> ETGLQPLPPTAFTPNGTYLQHLARDPTSGTLY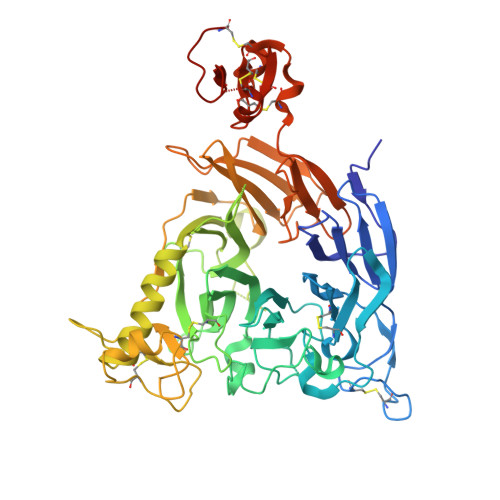LGATNFLFQLSPGLQLEATVSTGPVLDSRDCLPPVMPDECPQAQPTNNPNQLLLVSPGALVVCGSVHQGVCEQRRLGQLEQLLLRPERPGDTQYVAANDPAVSTVGLVAQGLAGEPLLFVGRGYTSRGVGGGIPPITTRALWPPDPQAAFSYEETAKLAVGRLSEYSHHFVSAFARGASAYFLFLRRDLQAQSRAFRAYVSRVCLRDQHYYSYVELPLACEGGRYGLIQAAAVATSREVAHGEVLFAAFSSAAPPTVGRPPSAAAGASGASALCAFPLDEVDRLANRTRDACYTREGRAEDGTEVAYIEYDVNSDCAQLPVDTLDAYPCGSDHTPSPMASRVPLEATPILEWPGIQLTAVAVTMEDGHTIAFLGDSQGQLHRVYLGPGSDGHPYSTQSIQQGSAVSRDLTFDGTFEHLYVMTQSTLLKVPVASCAQHLDCASCLAHRDPYCGWCVLLGRCSRRSECSRGQGPEQWLWSFQPELGCLQGTKHHHHHH We here present crystal structures of herring PGM5, the first structures of this protein from any species. PGM5 shows a bi-lobed structure with four domains arranged around a common active site, forming a deep cleft between domains I–II (residues 1–195 and 196–308) and domains III–IV (residues 309–425 and 426–567). As expected, all four domains contribute to the active site with one loop per domain; loop 1 (residues 119–126), loop 2 (residues 292–297), loop 3 (residues 379–384), and loop 4 (residues 507–520). Herring PGM5 binds substrate similarly to PGM1, but lacks enzymatic activity.

Furthermore, we have solved the structure of the most common PGM5 variants found in the Baltic and Atlantic herring (bPGM5 and aPGM5), differing by only one amino acid substitution (Ala330Val), and explore the possible functional significance of the mutation. Crystals of His6-tagged aPGM5 belong to space group P21, while crystals of His6-tagged bPGM5 belong to space group P21212, both with one molecule in the asymmetric unit. The aPGM5 structure consists of residues 4–567, except for residues 511–513. Despite crystallization of aPGM5 in a condition without divalent ions, a metal ion is observed in the active site, coordinated at around 2.4 Å distance by Asp292, Asp294, and Asp296 in loop 2. Due to the long coordination distances, the ion was modelled as calcium rather than magnesium. In aPGM5, Ser121 is unphosphorylated, suggesting that the phosphorylation state is batch-dependent. The structures of apo aPGM5 and bPGM5 are very similar (root mean square deviation (RMSD) of 0.64 Å over 545 Cα atoms), but aPGM5 is further closed, showing a shift of up to 2.4 Å of domain IV towards domain I. In contrast, aPGM5 did not crystallize in the same conditions but at other conditions formed small and irreproducible needle crystals in space group P21. Interestingly, Val330 is involved in a crystal contact in bPGM5, but the corresponding interface is not formed in the structure of aPGM5. The structures of aPGM5 and bPGM5 are overall very similar and even the backbone conformations at the mutation site are essentially identical.

> SMETNPIPVVTVQTTPFDDQKPGTNGLRKKTTVFESKKNYLQNYIQSVLSSIDLRDRQGCTMVVGSDGRYFSRTAIEVIVQMAAANGIGRLVIGHNGILSTPAVSCIIRKIKAIGGIILTASRNPGGPNGDFGIKFNVANGGPAPDTVIDKIHQVSRTLEEYAICPDMRIDLSRLGRQDFDLENKFKPFRVEIVDSVEVYLNLLRGIFDFNAIKGLLTGPDQLKMRVDAMSGVMGPYVRRILCDELGAPANSAVNCVPLEDFGGHYPDPNLTYATGLVDAMKGGEFGFGAAFDADGDRCMILGQNAFFVNPSDSLAVVAANLSCIPYFRQAGVRGFARSMPTSTAIDRVAKAMKVAVYETPAGWRFFGNLMDSGRCSFCGEESFGMGSDHIREKDGLWTVLVWLSIMAARKQGVEDIVRDHWTKLGRNYFCRFDYEAIDPRAAFYLMKDLEAVISDKAFCSQKFAVGNSVYSVEKADNFEYIDPVDGTVARNQGLRIIFSESSRLIFRLSGTGVGVGATIRIYAESFERDPERHNREPQVVLGPLIAIALKISDIHERTGRRGPTVIT>MAHTGRMFKIEAAEIVVARLPLKFRFETSFGVQTHKVVPLLILHGEGVQGVAEGTMEARPMYREETICGALCLLRGTFLPAILGQTFANPEAVSDALGSYRGNRMARAMVEMAAWDLWARTLGVPLGTLLGGHKEQVEVGVSLGIQADEQAT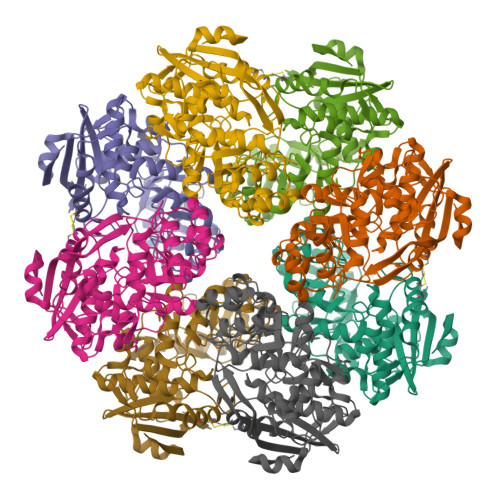VDLVRRHVEQGYRRIKLKIKPGWDVQPVRATREAFPDIRLTVDANSAYTLADAGRLRQLDEYDLTYIEQPLAWDDLVDHAELARRIRTPLCLDESVASASDARKALALGAGGVINLKVARVGGHAESRRVHDVAQSFGAPVWCGGMLESGIGRAHNIHLSTLSNFRLPGDTSSASRYWERDLIQEPLEAVDGLMPVPQGPGTGVTLDREFLATVTEAQEEHRA[4x]>MVNGDGNPREVIEDLAANNPAIQNIRLRHENKDLKARLENAMEVAGRDFKRAEELEKAKQALEDQRKDLETKLKELQQDYDLAKESTSWDRQRLEKELEEKKEALELAIDQASRDYHRATALEKELEEKKKALELAIDQASQDYNRAN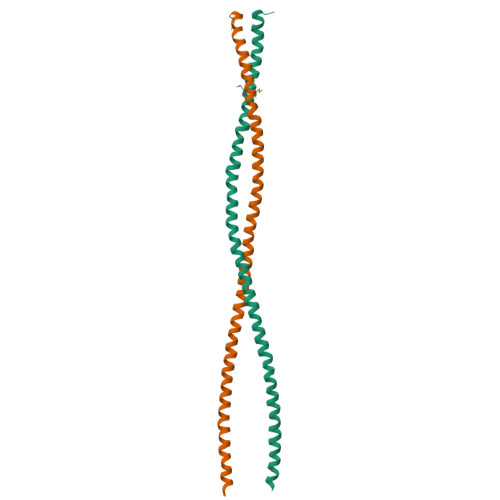VLEKELE[4x]> ALTCFSEGTKVPAWGCCPASWKSFGSSCYFISSEEKVWSKSEQNCVEMGAHLVVFNTEAEQNFIVQQLNESFSYFLGLSDPQGNNNWQWIDKTPYEKNVRFWHLGEPNHSA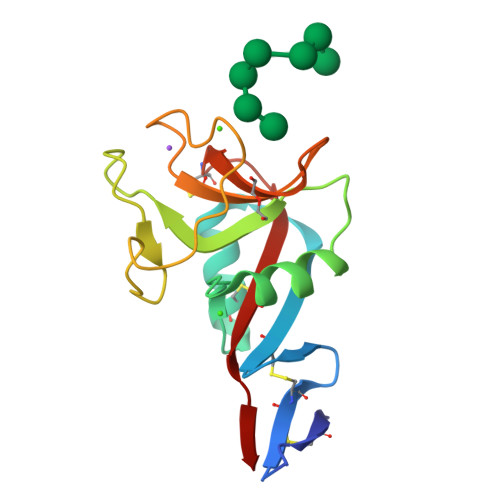EQCASIVFWKPTGWGWNDVICETRRNSICEMNKIYL> MTTTMKISIEFLEPFRMTKWQESTRRNKNNKEFVRGQAFARWHRNKKDNTKGRPYITGTLLRSAVIRSAENLLTLSDGKISEKTCCPGKFDTEDKDRLLQLRQRSTLRWTDKNPCPDNAETYCPFCELLGRSGNDGKKAEKKDWRFRIHFGNLSLPGKPDFDGPKAIGSQRVLNRVDFKSGKAHDFFKAYEVDHTRFPRFEGEITIDNKVSAEARKLLCDSLKFTDRLCGALCVIRFDEYTPAADSGKQTENVQAEPNANLAEKTAEQIISILDDNKKTEYTRLLADAIRSLRRSSKLVAGLPKDHDGKDDHYLWDIGKKKKDENSVTIRQILTTSADTKELKNAGKWREFCEKLGEALYLKSKDMSGGLKITRRILGDAEFHGKPDRLEKSRSVSIGSVLKETVVCGELVAKTPFFFGAIDEDAKQTDLQVLLTPDNKYRLPRSAVRGILRRDLQTYFDSPCNAELGGRPCMCKTCRIMRGITVMDARSEYNAPPEIRHRTRINPFTGTVAEGALFNMEVAPEGIVFPFQLRYRGSEDGLPDALKTVLKWWAEGQAFMSGAASTGKGRFRMENAKYETLDLSDENQRNDYLKNWGWRDEKGLEELKKRLNSGLPEPGNYRDPKWHEINVSIEMASPFINGDPIRAAVDKRGTDVVTFVKYKAEGEEAKPVCAYKAESFRGVIRSAVARIHMEDGVPLTELTHSDCECLLCQIFGSEYEAGKIRFEDLVFESDPEPVTFDHVAIDRFTGGAADKKKFDDSPLPGSPARPLMLKGSFWIRRDVLEDEEYCKALGKALADVNNGLYPLGGKSAIGYGQVKSLGIKGDDKRISRLMNPAFDETDVAVPEKPKTDAEVRIEAEKVYYPHYFVEPHKKVEREEKPCGHQKFHEGRLTGKIRCKLITKTPLIVPDTSNDDFFRPADKEARKEKDEYHKSYAFFRLHKQIMIPGSELRGMVSSVYETVTNSCFRIFDETKRLSWRMDADHQNVLQDFLPGRVTADGKHIQKFSETARVPFYDKTQKHFDILDEQEIAGEKPVRMWVKRFIKRLSLVDPAKHPQKKQDNKWKRRKEGIATFIEQKNGSYYFNVVTNNGCTSFHLWHKPDNFDQEKLEGIQNGEKLDCWVRDSRYQKAFQEIPENDPDGWECKEGYLHVVGPSKVEFSDKKGDVINNFQGTLPSVPNDWKTIRTNDFKNRKRKNEPVFCCEDDKGNYYTMAKYCETFFFDLKENEEYEIPEKARIKYKELLRVYNNNPQAVPESVFQSRVARENVEKLKSGDLVYFKHNEKYVEDIVPVRISRTVDDRMIGKRMSADLRPCHGDWVEDGDLSALNAYPEKRLLLRHPKGLCPACRLFGTGSYKGRVRFGFASLENDPEWLIPGKNPGDPFHGGPVMLSLLERPRPTWSIPGSDNKFKVPGRKFYVHHHAWKTIKDGNHPTTGKAIEQSPNNRTVEALAGGNSFSFEIAFENLKEWELGLLIHSLQLEKGLAHKLGMAKSMGFGSVEIDVESVRLRKDWKQWRNGNSEIPNWLGKGFAKLKEWFRDELDFIENLKKLLWFPEGDQAPRVCYPMLRKKDDPNGNSGYEELKDGEFKKEDRQKKLTTPWTPWA;> MSNPIRDIQDRLKTAKFDNKDDMMNLASSLYKYEKQLMDSSEATLCQQGLSNRPNSFSQLSQFRDSDIQSKAGGQTGKFWQNEYEACKNFQTHKERRETLEQIIRFLQNGAEEKDADDLLLKTLARAYFHRGLLYRPKGFSVPARKVEAMKKAIAYCEIILDKNEEESEALRIWLYAAMELRRCGEEYPENFAEKLFYLANDGFISELYDIRLFLEYTEREEDNNFLDMILQENQDRERLFELCLYKARACFHLNQLNDVRIYGESAIDNAPGAFADPFWDELVEFIRMLRNKKSELWKEIAIKAWDKCREKEMKVGNNIYLSWYWARQRELYDLAFMAQDGIEKKTRIADSLKSRTTLRIQELNELRKDAHRKQNRRLEDKLDRIIEQENEARDGAYLRRNPPCFTGGKREEIPFARLPQNWIAVHFYLNELESHEGGKGGHALIYDPQKAEKDQWQDKSFDYKELHRKFLEWQENYILNEEGSADFLVTLCREIEKAMPFLFKSEVIPEDRPVLWIPHGFLHRLPLHAAMKSGNNSNIEIFWERHASRYLPAWHLFDPAPYSREESSTLLKNFEEYDFQNLENGEIEVYAPSSPKKVKEAIRENPAILLLLCHGEADMTNPFRSCLKLKNKDMTIFDLLTVEDVRLSGSRILLGACESDMVPPLEFSVDEHLSVSGAFLSHKAGEIVAGLWTVDSEKVDECYSYLVEEKDFLRNLQEWQMAETENFRSENDSSLFYKIAPFRIIGFPAE

The type III-E CRISPR-Cas system is a newly identified bifunctional complex with nuclease activity and protease activity that holds great potential for RNA editing applications. Here, we report cryo-electron microscopy (cryo-EM) structures of Desulfonema ishimotonii (Di) Cas7-11-crRNA, complexed with or without the full length or the N-terminus of TPR-CHAT. The Cas7 domains, arranged in a row, form a crescent-shaped filament, with the INS and CTE domain completing the structure. The Cas11 domain is positioned at the crescent’s midpoint, and interacts with Cas7.2 and Cas7.3.

DiTPR-CHAT consists of two main components: the NTD (amino acid residues 1–65) and the CTD (amino acid residues 75–751). The TPR domain of DiTPR-CHAT spans from Cas7.1 to Cas7.4, while the CHAT protease domain is close to Cas7.1 and Cas7.2. The NTD interacts with Cas7.4 primarily through hydrogen bonds, salt bridges, and nonbonded contacts. Indeed, the structure of DiCas7-11-crRNA-TPR-CHAT also exhibits interactions between L2 and CHAT domains in additional to those in the NTD, which explains the stabilized conformation of L2 observed in the structure. Structural analysis revealed that the binding of DiTPR-CHAT did not induce significant conformational changes in the overall configuration of DiCas7-11-crRNA complex, but it did stabilize the conformations in the L2 and Cas7.4 regions. Further analysis demonstrated that DiTPR-CHAT, primarily via its NTD, maintained the stable conformation of DiCas7-11-crRNA by establishing multiple interactions with Cas7.4. This contributed to the prevention of target RNA binding to the crRNA and resulted in reduced cleavage activity. Numerous studies have conducted functional characterizations of the residues that interact with the crRNA in this region, highlighting the essential nature of some amino acid residues for pre-RNA processing. Importantly, in the TPR-CHAT bound structure, the crRNA-binding region retained conformation and exhibited no contact with TPR-CHAT, indicating that pre-crRNA processing is not mediated by DiTPR-CHAT. We found that DiCas7-11-crRNA specifically cleaved the target RNA into two fragments, and the presence of DiTPR-CHAT inhibited this cleavage. We found that the affinity of the DiCas7-11-crRNA complex to the target RNA was reduced by the presence of full length (F) or NTD of DiTPR-CHAT but unaffected by the CTD.>[2x]ANDSPAKSLVDIDLSSLRDPAGIFELVEVVGNGTYGQVYKGRHVKTGQLAAIKVMDVTEDEEEEIKLEINMLKKYSHHRNIATYYGAFIKKSPPGHDDQL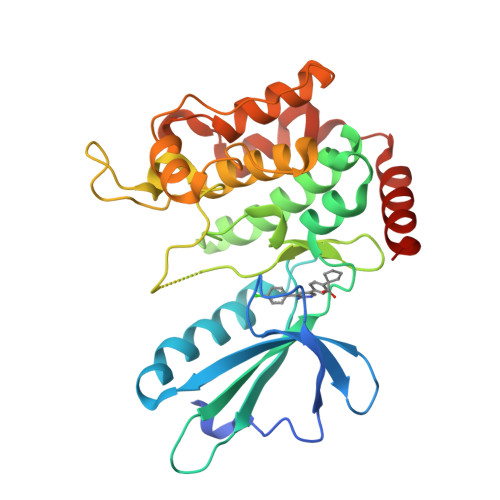WLVMEFCGAGSITDLVKNTKGNTLKEDWIAYISREILRGLAHLHIHHVIHRDIKGQNVLLTENAEVKLVDFGVSAQLDRTVGRRNTFIGTPYWMAPEVIACDENPDATYDYRSDLWSCGITAIEMAEGAPPLCDMHPMRALFLIPRNPPPRLKSKKWSKKFFSFIEGCLVKNYMQRPSTEQLLKHPFIRDQPNERQVRIQLKDHIDRTRKKR> MDKLLERFLHYVSLDTQSKSGVRQVPSTEGQWKLLRLLKQQLEEMGLVNITLSEKGTLMATLPANVEGDIPAIGFISHVDTSPDFSGKNVNPQIVENYRGGDIALGIGDEVLSPVMFPVLHQLLGQTLITTDGKTLLGADDKAGVAEIMTALAVLKGNPIPHGDIKVAFTPDEEVGKGAKHFDVEAFGAQWAYTVDGGGVGELEFENFNAASVNIKIVGNNVHPGTAKGVMVNALSLAARIHAEVPADEAPETTEGYEGFYHLASMKGTVDRAEMHYIIRDFDRKQFEARKRKMMEIAKKVGKGLHPDCYIELVIEDSYYNMREKVVEHPHILDIAQQAMRDCHITPEMKPIRGGTDGAQLSFMGLPCPNLFTGGYNYH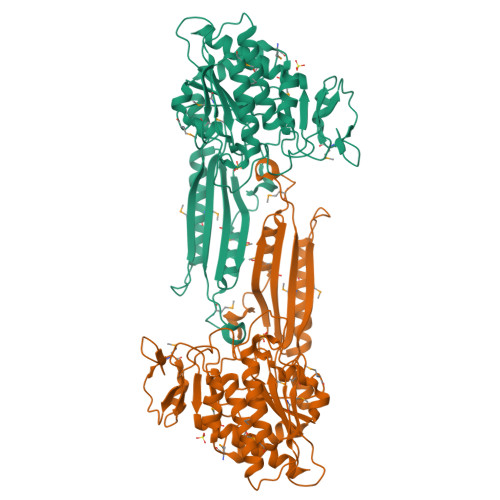GKHEFVTLEGMEKAVQVIVRIAELTAKRGQLEHHHHHH>SRNFIIPKKEIHTVPDMGKWKRSQAYADYIGFILTLNEGVKGKKLTFEYRVSEAIEKLVALLNTLDRWIDETPPVDQPSRFGNKAYRTWYAKLDEEAENLVATVVPTHLAAAVPEVAVYLKESVGNSTRIDYGTGHEAAFAAFLCCLCKIGVLRVDDQIAIVFKVFNRYLEVMRKLQKTYRMEPAGSQGVWGLDDFQFLPFIWGSSQLIDHPYLEPRHFVDEKAVNENHKDYMFLECILFITEMKTGPFAEHSNQLWNISAVPSWSKVNQGLIRMYKAEC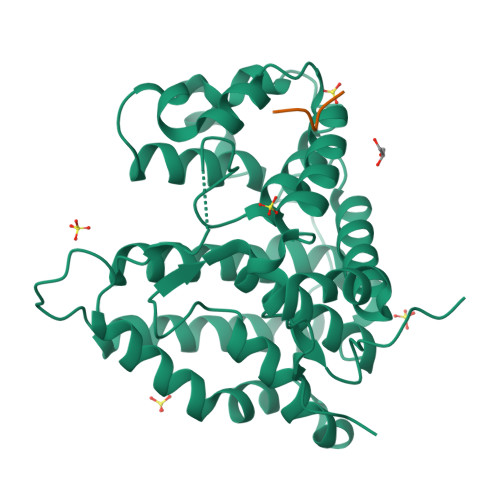LEKFPVIQHFKFGSLLPIHPVTSG[2x];>[2x]TPDYFL>[4x]MVLMIVSGRSGSGKSVALRALEDMGFYCVDNLPVVLLPDLARTLADR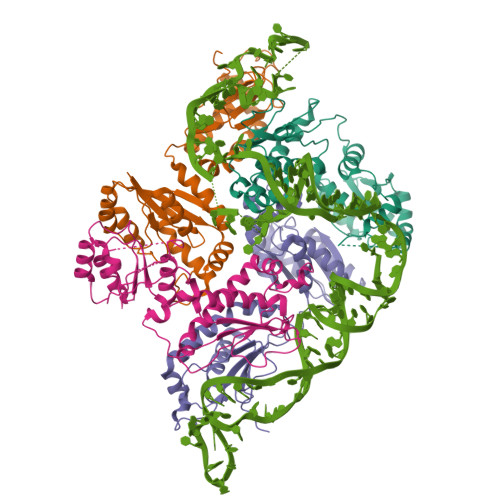EISAAVSIDVRNMPESPEIFEQAMSNLPDAFSPQLLFLDADRNTLIRRYSDTRRLHPLSSKNLSLESAIDKESDLLEPLRSRADLIVDTSEMSVHELAEMLRTRLLGKRERELTMVFESFGFKHGIPIDADYVFDVRFLPNPHWDPKLRPMTGLDKPVAAFLDRHTEVHNFIYQTRSYLELWLPMLETNNRSYLTVAIGCTGGKHRSVYIAEQLADYFRSRGKNVQSRHRTLEKRKP> GMLKNDQLDQWDRDNFFHPSTHLAQHARGESANRVIKTASGVFIEDRDGTKLLDAFAGLYCVNVGYGRQEIAEAIADQARELAYYHSYVGHGTEASITLAKMILDRAPKNMSKVYFGLGGSDANETNVKLIWYYNNILGRPEKKKIISRWRGYHGSGLVTGSLTGLELFHKKFDLPVEQVIHTEAPYYFRREDLNQTEEQFVAHCVAELEALIER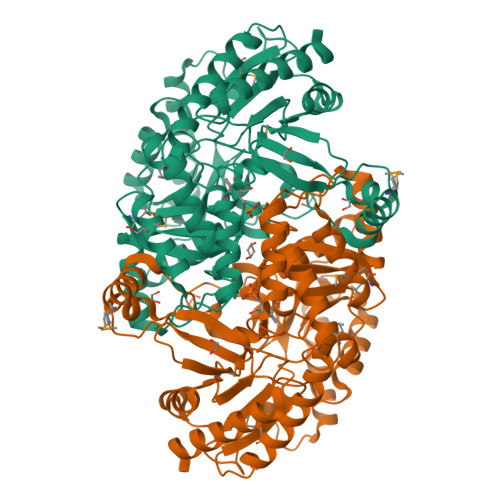EGADTIAAFIGEPILGTGGIVPPPAGYWEAIQTVLNKHDILLVADEVVTGFGRLGTMFGSDHYGLEPDIITIAKGLTSAYAPLSGSIVSDKVWKVLEQGTDENGPIGHGWTYSAHPIGAAAGVANLKLLDELNLVSNAGEVGAYLNATMAEALSQHANVGDVRGEGLLCAVEFVKDRDSRTFFDAADKIGPQISAKLLEQDKIIARAMPQGDILGFAPPFCLTRAEADQVVEGTLRAVKAVLG>AEKEKNAAEIRQQFAMTAGSPIIVNDKLERYAEVRTAFTHPTSFFKPNYKGEVKPWFLSAYDEKVRQIENGENGPKMKAKNVGEARAGRALEAAGWTLDINYGNIYPNRFFMLWSGETMTNTQLWAPVGLDRRPPDTTDPVELTNYVKFAARMAGADLVGVARLNRNWVYSEAVTIPADVPYEQSLHKEIEKPIVFKDVPLPIETDDELIIPNTCENVIVAGIAMNREMMQTAPNSMACATTAFCYSRMCMFDMWLCQF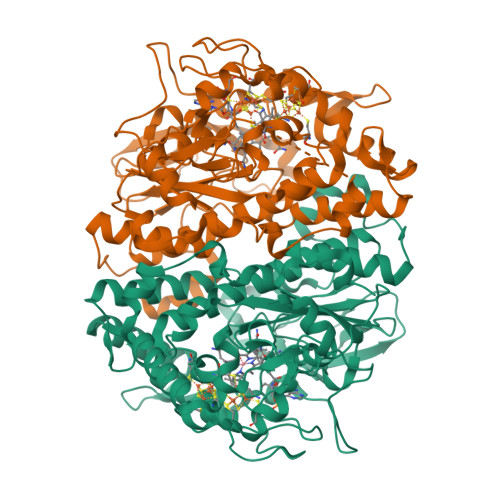IRYMGYYAIPSCNGVGQSVAFAVEAGLGQASRMGACITPEFGPNVRLTKVFTNMPLVPDKPIDFGVTEFCETCKKCARECPSKAITEGPRTFEGRSIHNQSGKLQWQNDYNKCLGYWPESGGYCGVCVAVCPFTKGNIWIHDGVEWLIDNTRFLDPLMLGMDDALGYGAKRNITEVWDGKINTYGLDADHFRDTVSFRKDRVKKS[6x]>MDFNLSNSQSDIYESAYRFACDVLDQDAQTRISQKILSTELWKKAAAYGF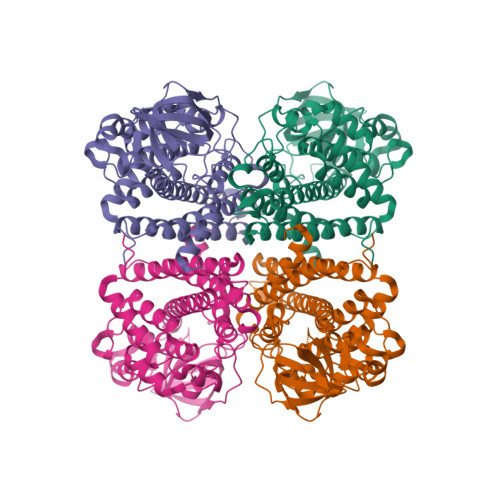AHGPVSHQFGGSELGALDTALMIEALGKGSRDIGLSFSLCAHLCACVIPLYRFGSSELKDKYLESLVTGKLIAANAATEPDAGSDIYNMQATAQPCEGGYILNGKKIFITNAPIADVFIIYAKTNPDHGFLGVSAFLIEKGTPGLNVGEVIPKDCLSNCPWSEIVFNDIFIPQSQRIGMEGAGGAIFHDSMIWEKGCLSALFVGGLARLLETTLEYAKARQQFGKAIGQFQSVSNRIIDMKLRLEQCRLMLYRACWKHDQGQDAEADIAMSKLLISEYAVQSGLDAIQTFGGAAMDQELGLVRHLLNMIPSRIFSGTNDIQKEIIARKLGLRGTSSGSLVPRGSHHHHHHHH[2x]>[2x]MFENEILFDNGQHKFMFLGWEEKEEEIVQTNQYLILDGNEGILLDPGGAHVFPRVMSNVA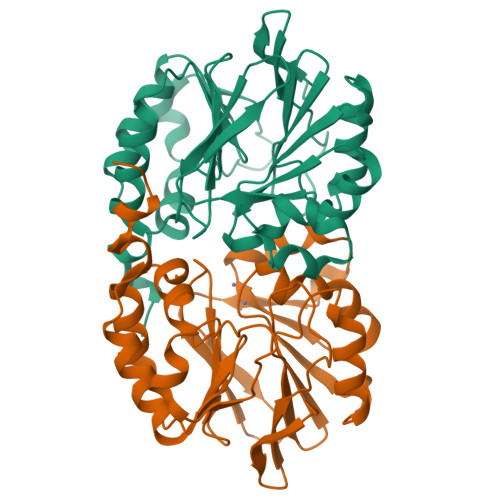EVVDLSSIRHIFYTHQDPDVTSGILLWLSICENAKIYISSLWVRFLPHFGIYDQKRIVPISDKGTKIKLLSGNELEILPAHFLHSTGNFVLYDPVAKILFSGDIGAAVFEKGKRYRYVDDFERHLPLMEAFHKRYMSSNAACKKWVDMVSKKKIDMIAPQHGAVFRGESVKKFLEWFRNLKCGVDLIDNLYSL>[4x]MGQGDESERIVINVGGTRHQTHRSTLRTLPGTRLAWLAEPDAHSHFDYDPRADEFFFDRHPGVFAHILNYYRTGKLHCPADVCGPLYEEELAFWGIDETDVEPCCWMTYRQHRDAEEALDSFGGAPLDNSADDADADGPGDSGDGEDELEMTKRLALSDSPDGRPGGFWRRWQPRIWALFEDPYSSRYARYVAFASLFFILVSITTFCLETHERFNPIVNKTEIENVRNGTQVRYYREAETEAFLTYIEGVCVVWFTFEFLMRVIFCPNKVEFIKNSLNIIDFVAILPFYLEVGLSGLSSKAAKDVLGFLRVVRFVRILRIFKLTRHFVGLRVLGHTLRASTNEFLLLIIFLALGVLIFATMIYYAERIGAQPNDPSASEHTHFKNIPIGFWWAVVTMTTLGYGDMYPQTWSGMLVGALCALAGVLTIAMPVPVIVNNFGMYYSLAMAKQKLPKKKKKHIPRPPQLGSPNYCKSVVNSPHHSTQSDTCPLAQEEILEINRAGRKPLRGMSIAENLYFQ

Voltage-gated K+ channels of the Kv3 family represent an important subfamily among the 70 different Kv channel genes in the human genome, with specialized biophysical properties to sustain high-frequency firing of action potentials. The combination of ultra-fast activation and deactivation kinetics and high activation potential of these channels are key for their ability to repolarize the membrane and terminate the action potential. Like other pore-forming subunits of Kv channels, Kv3 members are comprised of an N-terminal cytoplasmic T1 domain, which is involved but not required for Zn2+-mediated tetramerization, followed by the voltage-sensing domain (VSD) with transmembrane helices S1–S4 which is connected via a helical linker (S4/S5L) to the pore forming domain (PD) of the channel. Here, we present cryo-EM structures of the human Kv3.1a channel in an activated state, providing mechanistic insights into the modulation of Kv3 channels by the cytoplasmic T1 domain.

To elucidate the structural determinants underlying the biophysical properties of Kv3 channels, we purified the shorter α-isoform of Kv3.1 from mammalian cells and determined cryo-EM structures under different sample conditions (apo, Zn2+-containing vs. Zn2+-free). We achieved 3D reconstructions between 3.1 and 3.5 Å for the different conditions, which show only minor differences in the overall structure, and no clear densities for additional Zn2+ sites other than the known sites in the T1 domain16 (see Supplementary discussion). In the following structural analysis, we thus focus mostly on observations from the best resolved structure which was obtained in digitonin and in the presence of 400 μM Zn2+ (representative densities for different regions of the channel are shown in Fig. S4). When superposing the TM region of Kv3.1a with the respective region in the structure of the Kv1.2-Kv2.1 chimera, the T1 domain of Kv3.1a is rotated clockwise by ~48° with respect to the T1 domain of Kv1.2-2.1. As a result of these differences, the α6 helix in the context of the full Kv3.1a channel is rotated by an almost 90° angle compared to Kv1.2-2.1, bringing it in much closer proximity to the S4/S5 linker. Consistent with the high activation potential of Kv3.1, the S4 helix of the VSD is in a less activated conformation compared to Kv1.2/Kv2.1 and Kv4.2, with only three (R1–R3) of the four voltage-sensing charges located above the conserved F256 in S2, which is part of the hydrophobic charge transfer centre (CTC) defined in previous Kv channel structures. Despite the less activated S4 position in the VSDs, the lower S6 gate of Kv3.1 is captured in a dilated conformation, exhibiting a pore radius near the PVP region large enough to accommodate a hydrated K+ ion. In addition to the zinc-coordinating interactions of C104/C105 in α6 and H77 in the α4/α5 linker, two acidic residues (E116 and D120) at the C-terminal end of α6 are forming salt bridges to K449 in S6T.> MGHHHHHHAMANDTEDIGKGSDIEIIKRTEDKTSNKWGVTQNIQFDFVKDKKYNKDALILKMQGFISSRTTYYNYKKTNHVKAMRWPFQYNIGLKTNDKYVSLINYLPKNKIESTNVSQTLGYNIGGNFQSAPSLGGNGSFNYSKSISYTQQNYVSEVEQQNSKSVLWGVKANSFATESGQKSAFDSDLFVGYKPHSKDP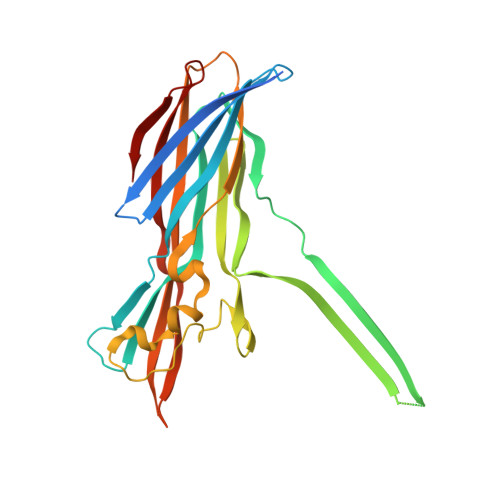RDYFVPDSELPPLVQSGFNPSFIATVSHEKGSSDTSEFEITYGRNMDVTHAIKRSTHYGNSYLDGHRVHNAFVNRNYTVKYEVNWKTHEIKVKGQN> AEVGRLRYPPEMPGAEVKVYKKVDNVDLKLYIYKPADWKPADRRSAIVFFFGGGWQSGSPAQFRPQCEYFAGRGMVAMAADYRVGSRHNVKVADCVADAKSAIRWVRQHAAELGVDPQKIVASGGSAGG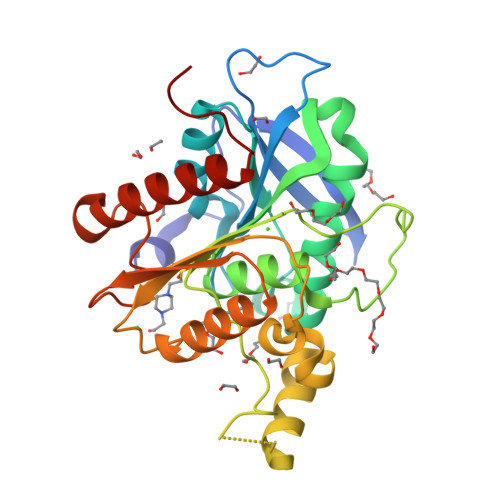HLAACTVMVPDLEAPEEDHTISSQANAAILFNPVLILSREGLKDHVPRQDWEERLRERLGTEPKAVSPYHHIRAGLPPMIIFHGTADNTVPFETIRLFAEAMKKAGNRCELVPFEGAAHGFFNFGRGDNLAYQKTLELADEFLVEIGFLAPKGESQP> AASXDXSLVEVHXXVFIVPPXILQAVVSIATTRXDDXDSAAASIPMVPGWVLKQVXGSQAGSFLAIVMGGGDLEVILIXLAGYQESSIXASRSLAASMXTTAIPSDLWGNXAXSNAAFSSXEFSSXAGSVPLGFTFXEAGAKEXVIKGQITXQAXAFSLAXLXKLISAMXNAXFPAGDXXXXVADIXDSHGILXXVNYTDAXIKMGIIFGSGVNAAYWCDSTXIADAADAGXXGGAGXMXVCCXQDSFRKAFPSLPQIXYXXTLNXXSPXAXKTFEKNSXAKNXGQSLRDVLMXYKXXGQXHXXXAXDFXAANVENSSYPAKIQKLPHFDLRXXXDLFXGDQGIAXKTXMKXVVRRXLFLIAAYAFRLVVCXIX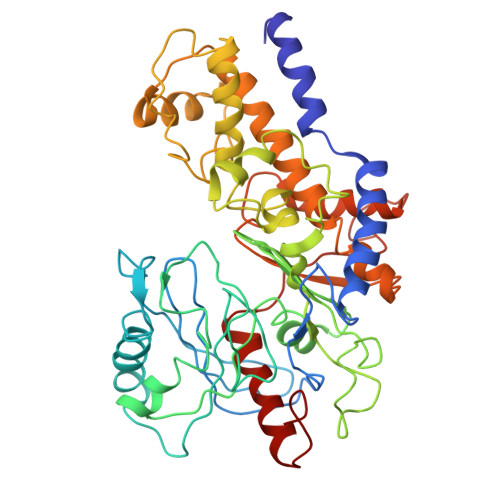AICQKKGYSSGHIAAXGSXRDYSGFSXNSATXNXNIYGWPQSAXXSKPIXITPAIDGEGAAXXVIXSIASSQXXXAXXSAXXA> MKNDKKVVVKV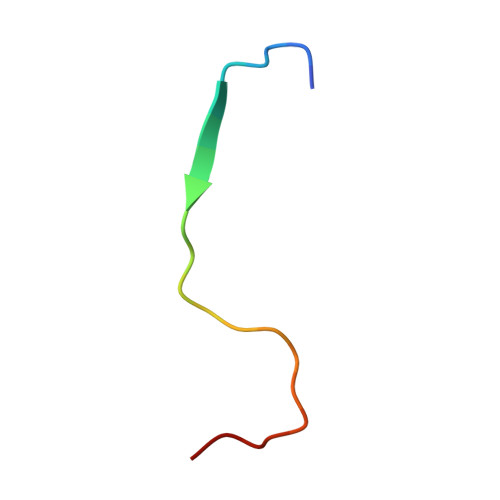KDKEMTCGAFN>[6x]MGSSHHHHHHSSGLVPAGSHSKVFIRSAINRVHQNSAANGGELPRIVFPEGTSTKVLKALATLVEEKICQPILLGYPERVKEKIKALDIPLLNDVSIVHPSSHPKYFSFVEKLYSLAQRKGINLGEAERLMADPNYFAAMMVNQGEADGMVSGSSINYADAVRPILQTIGVY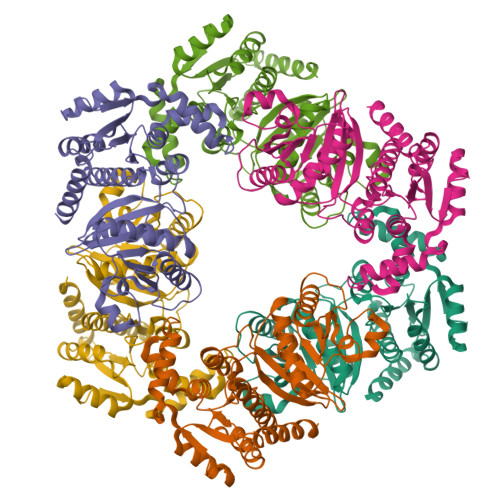KEGIPAGLNFVLLEDKFLVLADTTVNLNPTAEQCAQIALQAAKIVEYFGIEPRVAMLSYSNFSGAEGTPRKMKKAAEIARSLRPDLMIEGDMQADTAVNPEIMERLFPFSGLKGGANVLVFPNLESSNIAYKLIQQIGKAEVIGPFLTGVRRSANVLQRTTTVDGIVNSVVFTALEAQYIKEVLKSRGKK N-(4-NITROPHENYL)-2-PHENYL-THIOMORPHOLINE-4-CARBOXAMIDE | C17 H17 N3 O3 S | 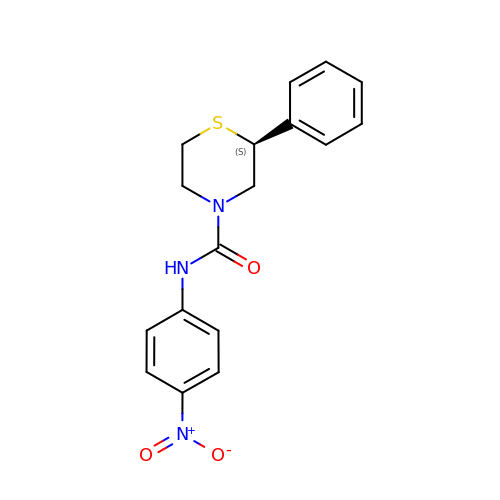PNYRURHCCDDZLP-MRXNPFEDSA-N>MSLHSDESNWQTFKRLWTYIRLYKAGLVVSTIALVINAAADTYMISLLKPLLDEGFGNAESNFLRILPFMILGLMFVRGLSGFASSYCLSWVSGNVVMQMRRRLFNHFMHMPVRFFDQESTGGLLSRITYDSEQVAGATSRALVSIVREGASIIGLLTLMFWNSWQLSLVLIVVAPVVAFAISFVSKRFRKISRNMQTAMGHVTSSAEQMLKGHKVVLSYGGQEVERKRFDKVSNSMRQQTMKLVSAQSIADPVIQMIASLALFAVLFLASVDSIRAELTPGTFTVVFSAMFGLMRPLKALTSVTSE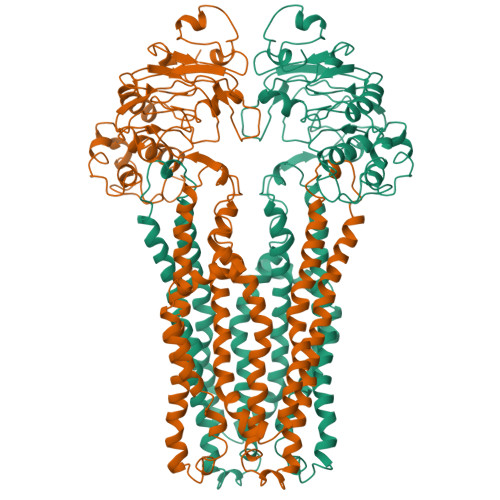FQRGMAACQTLFGLMDLETERDNGKYEAERVNGEVDVKDVTFTYQGKEKPALSHVSFSIPQGKTVALVGRSGSGKSTIANLFTRFYDVDSGSICLDGHDVRDYKLTNLRRHFALVSQNVHLFNDTIANNIAYAAEGEYTREQIEQAARQAHAMEFIENMPQGLDTVIGENGTSLSGGQRQRVAIARALLRDAPVLILDEATSALDTESERAIQAALDELQKNKTVLVIAHRLSTIEQADEILVVDEGEIIERGRHADLLAQDGAYAQLHRIQFGE[2x]>[4x]PEIITPIITPFTKDNRIDKEKLKIHAENLIRKGIDKLFVNGTTGLGPSLSPEEKLENLKAVYDVTNKIIFQVGGLNLDDAIRLAKLS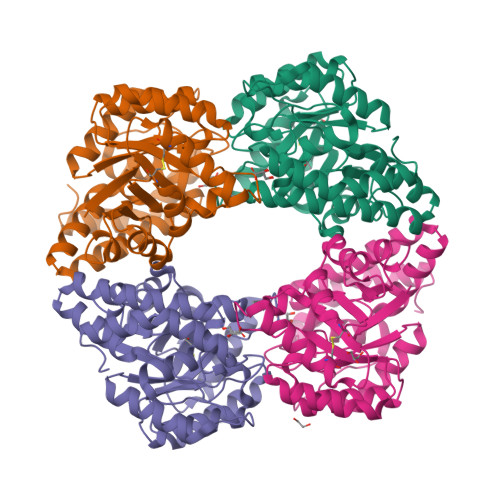KDFDIVGIASYAPYYYPRMSEKHLVKYFKTLCEVSPHPVYLYNYPTATGKDIDAKVAKEIGCFTGVKDVIENIIHTLDYKRLNPNMLVYSGSQMLIATVASTGLDGNVALGSNYLPEVTVTIKKLAMERKIDEALKLQFLHDEVIEASRIFGSLSSNYVLTKYFQGYDLGYPRPPIFPLDDEEERQLIKKVEGIRAKLVELKILKE> QIGWRREGIKYRRNELFLDVLESVNLLMSPQGQVLSAHVSGRVVMKSYLSGMPECKFGMNDKIVIEX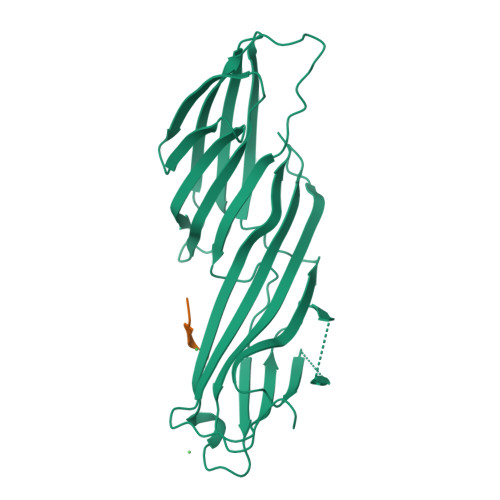XXXXXXXXXXXXXXXXXXXXXXXXXXXXXXXXXXXXRSISFIPPDGEFELMRYRTTKDIILPFRVIPLVREVGRTKLEVKVVIKSNFKPSLLAQKIEVRIPTPLNTSGVQVICMKGKAKYKASENAIVWKIKRMAGMKESQISAEIELLPTNDKKKWARPPISMNFEVPFAPSGLKVRYLKVFEPKLNYSDHDVIKWVRYIGRSGIYETRC;> GYMPMSPG>MPHIRVRGAEKEKVRDFTAGLADELGIIAECPADWFTFEYVETTFFFDGKEDDGLVFIEVLWF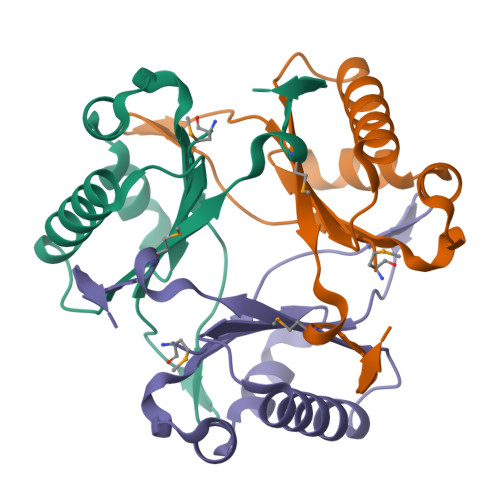DRDSEARDKIAALFTERWKKITDKIVTIVFNPLIENMYYEDGVHFAENLYFQGHHHHHHHHHH[2x]> AEQGPSLLQNKCMGCHIPEGNDTYSRISHQRKTPEGWLMSIARMQVMHGLQISDDDRRTLVKYLADKQGLAPSETDGVRYAM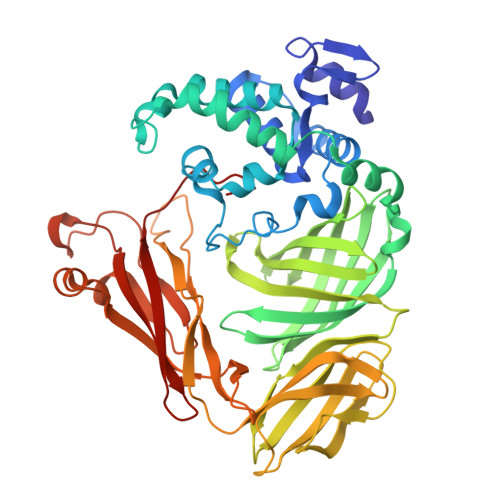ERRLNTVEQFDTQLSETCGRCHSGARVALQRRPAKEWEHLVNFHLGQWPSLEYQAQARDRDWLPIALQQVVPDLAKRYPLESAAWAEWQKARPKADALPGQWAFSGHMLAKGDVRGVMSVTPDQGDTFKVEVKGAYADGTPFNGSGSAILYNGYEWRGNVKVGDANLRQVFAALDGEMKGRMFEAEHDERGLDFTAVKEGKARLLAVQPAFIKAGGESEITLVGSGLAGKPDLGAGVEVTEVLEQTPTLVRLKARAAADAKPGQREVAVGTLKGVNLAVYDKVEEVKVVPAFSIARIGENGASVPKVQGRFEAEAWGKDANGQPLRIGYLPASWKVEPFNERAVEDEDVKFAGKMQADGVFVPGGAGPNPERKMMTNNAGNLKVIATLADGGQTGEGHMIVTVQRWNNPPLP> MGSSHHHHHSSGLVPRGSHMSKDSDYKRAEKHLSSIDNKWSSLVKKVGPCTLTPHPEHAPYEGIIRAITSQKLSDAATNSIINKFCTQCSDNDEFPTPKQIMETDVETLHECGFSKLKSQEIHIVA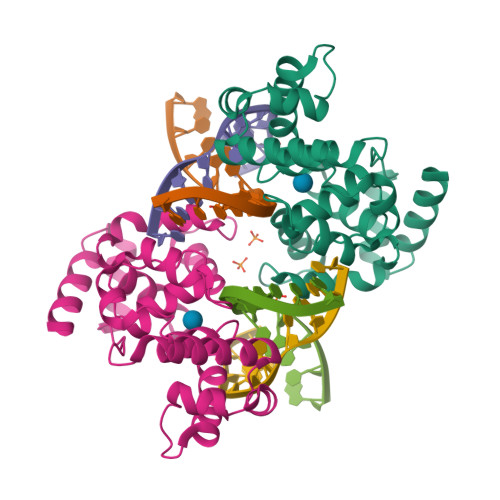EAALNKQIPSKSEIEKMSEEELMESLSKIKGVKRWTIEMYSIFTLGRLDIMPADDSTLKNEAKEFFGLSSKPQTEEVEKLTKPCKPYRTIAAWYLWQIPKLHRKGQ>[2x]SNAVLKIIQGALDTRELLKAYQEEACAKNFGAFCVFVGIVRKEDNIQGLSFDIYEALLKTWFEKWHHKAKDLGVVLKMAHSLGDVLIGQSSFLCVSMGKNRKNALELYENFIEDFKHNAPI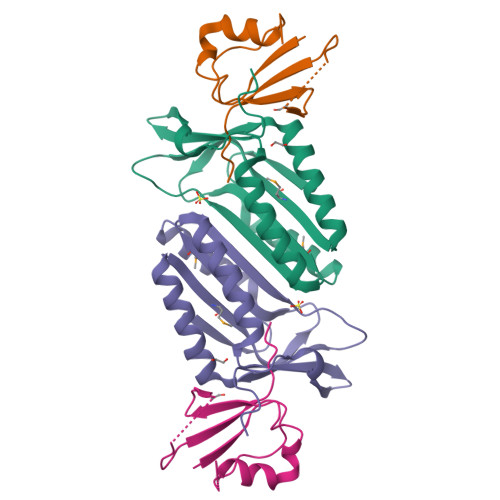WKYDLIHNKRIYAKERSHPLKGSGLLA;>[2x]MMVEVRFFGPIKEENFFIKANDLKELRAILQEKEGLKEWLGVCAIALNDHLIDNLNTPLKDGDVISLLPPVCGG>SHMLRPVETPTREIKKLDGLWAFSLDRENCGIDQRWWESALQESRAIAVPGSFNDQFADADIRNYVGNVWYQREVFIPKGWAGQRIVLRFDAVTHYGKVWVNNQEVMEHQGGYTPFEADVTPYVIAGKSVRITVCVNNELNWQTIPPGMVITDENGKKKQSYFHDFFNYAGIHRSVMLYTTPNTWVDDITVVTHVAQDCNHASVDWQVVANGDVSVELRDADQQVVATGQGTSGTLQVVNPHLWQPGEGYLYELCVTAKSQT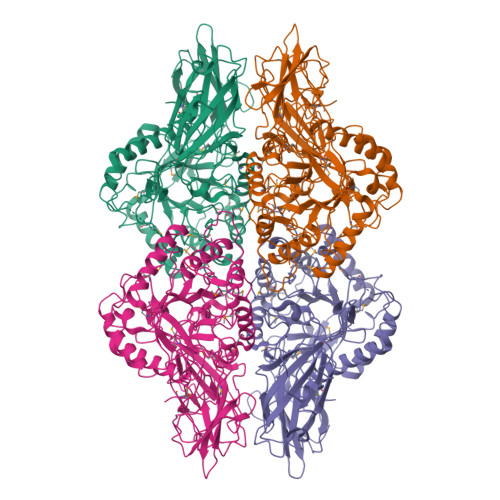ECDIYPLRVGIRSVAVKGEQFLINHKPFYFTGFGRHEDADLRGKGFDNVLMVHDHALMDWIGANSYRTSHYPYAEEMLDWADEHGIVVIDETAAVGFNLSLGIGFEAGNKPKELYSEEAVNGETQQAHLQAIKELIARDKNHPSVVMWSIANEPDTRPQGAREYFAPLAEATRKLDPTRPITCVNVMFCDAHTDTISDLFDVLCLNRYYGWYVQSGDLETAEKVLEKELLAWQEKLHQPIIITEYGVDTLAGLHSMYTDMWSEEYQCAWLDMYHRVFDRVSAVVGEQVWNFADFATSQGILRVGGNKKGIFTRDRKPKSAAFLLQKRWTGMNFGEKPQQGGKQ[2x]>ASSIKTPEDIEKMRVAGRLAAEVLEM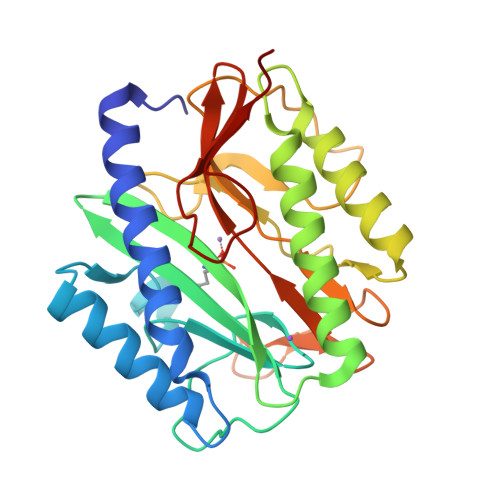IEPYVKPGVSTGELDRICNDYIVNEQHAVSACLGYHGYPKSVCISINEVVCHGIPDDAKLLKDGDIVNIDVTVIKDGFHGDTSKMFIVGKPTIMGERLCRITQESLYLALRMVKPGINLREIGAAIQKFVEAEGFSVVREYCGHGIGRGFHEEPQVLHYDSRETNVVLKPGMTFTIEPMVNAGKKEIRTMKDGWTVKTKDRSLSAQYEHTIVVTDNGCEILTLRKDDTIPAIISHDE[2x]>[2x]MLLNRANSTDSLSFSFINFDRDERNLIFQGDAHTSRNNILQLTRTDSNGAPVRSTVGRILHSAQVRLWEKSTNRVANLQTQFSFFLSSPLSNPADGIAFFIAPPDTTIPSGSAGGLLGLFNPRTALNESANQVLAVEFDTFFAQNSNTWDPNY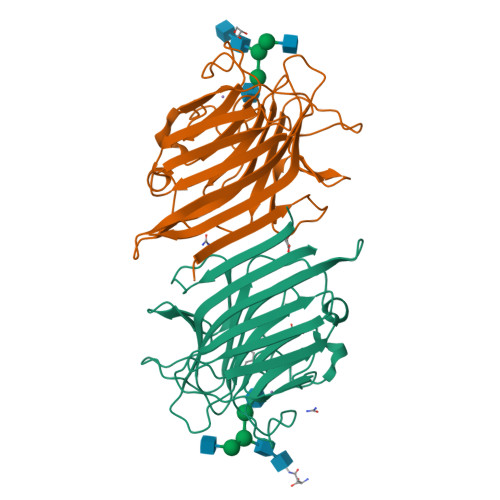QHIGIDVNSIRSSKVVRWERREGKTLNVLVTYNPSTRTIDVVATYPDGQRYQLSHVVDLTTILPEWVRVGFSAASGEQFQTHNLESWSFTSTLLYTAQKEDEYLARDM Hence, this loss of critical proteins has the potential to compromise ER proteostasis and generate cellular stress. This challenge to normal metabolism is overcome by the activity of the cytosolic coatomer protein I (COPI) polymer, whose repeating unit is the coatomer, a 560 kDa complex of seven distinct gene products (α-, β-, β′-, γ-, δ-, ε-, and ζ-COPI)25–31. Overall, the coatomer functions to retrieve the escaped “client” proteins, such as type I membrane proteins, from cis-Golgi back to ER by retrograde trafficking. In particular, the S protein – a type I membrane protein – is delivered to the ERGIC from both the ER (by anterograde trafficking) and the Golgi (by retrograde trafficking)3,10–12. Here we utilize recombinant SARS-CoV-2 S proteins and tail peptides, including constructs with enhanced mimicry of the coatomer binding motif (clientized S protein), to elucidate the atomic structure of the S-coatomer interface.

To determine an atomic-level understanding of S-coatomer interactions, we attempted co-crystallization of αWD40 with either wild-type (1267Gly-Val-Lys-Leu-His-Tyr-Thr1273) or clientized (1267Gly-Val-Lys-Leu-His-Tyr-Glu1273) S tail heptapeptides. However, in our co-crystallization experiments, contacts between symmetry-related αWD40 molecules occluded the binding site and no S tail peptide density was observed. Hence, we subsequently adopted a previously described strategy of using β‘WD40 for co-crystallization of peptides containing the Lys-x-His-x-xCT motif 61, which was also used for structural investigations of S tail peptides, recently during the revision of this manuscript. The β‘WD40 co-crystal structures with the wild-type and clientized Thr127Glu S heptapeptides were determined to a resolution of 1.4 Å. Overall, these two crystal structures reveal substantial similarity (Cα RMSD = 0.2 Å). The S tail heptapeptides are intercalated between two stacked β‘WD40 domains. The S tail extended motif makes contact with the binding site residues in one of the two β‘WD40 domains whereas the upstream tail residues interact with the other β‘WD40 domain, but at the face distal from the binding site. The major difference is that whereas only the main chain carboxylate of wild-type Thr1273 interacts with basic Lys17 on the β‘WD40 surface, both the side chain and main chain carboxylate groups of the clientized Glu1273 residue form extensive interactions with a β’WD40 basic cluster of Arg15, Lys17, and Arg272. This suggests that interactions between Glu1273 and the basic cluster underlie the enhanced binding of the clientized S protein. Overall, the two heptapeptides occupy the canonical WD40 binding site, which provides electrostatic complementarity to the dibasic motif residues, Lys1269 and His1271. B Glu1273 in clientized S forms complementary electrostatic interactions with the β‘WD40 basic cluster.

>SMKLDIKKTFSNRSDRVKGIDFHPTEPWVLTTLYSGRVEIWNYETQVEVRSIQVTETPVRAGKFIARKNWIIVGSDDFRIRVFNYNTGEKVVDFEAHPDYIRSIAVHPTKPYVLSGSDDLTVKLWNWENNWALEQTFEGHEHFVMCVAFNPKDPSTFASGCLDRTVKVWSLGQSTPNFTLTTGQERGVNYVDYYPLPDKPYMITASDDLTIKIWDYQTKSCVATLEGHMSNVSFAVFHPTLPIIISGSEDGTLKIWNSSTYKVEKTLNVGLERSWCIATHPTGRKNYIASGFDNGFTVLSLG[2x];>GVKLHYE[2x]>[2x]MNPAAEAEFNILLATDSYKVTHYKQYPPNTSKVYSYFECREKKTENSKLRKVKYEETVFY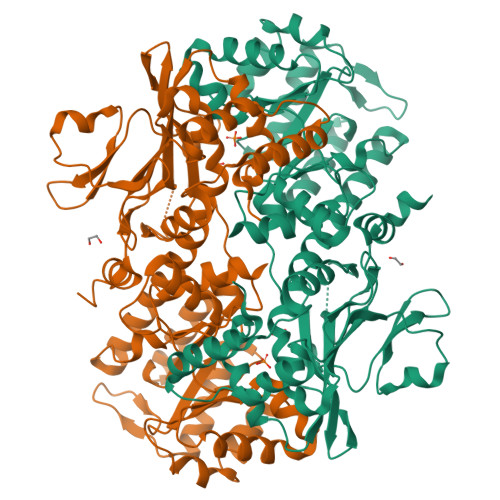GLQYILNKYLKGKVVTKEKIQEAKDVYKEHFQDDVFNEKGWNYILEKYDGHLPIEIKAVPEGFVIPRGNVLFTVENTDPECYWLTNWIETILVQSWYPITVATNSREQKKILAKYLLETSGNLDGLEYKLHDFGYRGVSSQETAGIGASAHLVNFKATDTVAGLALIKKYYGTKDPVPGYSVPAAEHSTITAWGKDHEKDAFEHIVTQFSSVPVSVVSDSYDIYNACEKIWGEDLRHLIVSRSTQAPLIIRPDSGNPLDTVLKVLEILGKKFPVTENSKGYKLLPPYLRVIQGDGVDINTLQEIVEGMKQKMWSIENIAFGSGGGLLQKLTRDLLNCSFKCSYVVTNGLGINVFKDPVADPNKRSKKGRLSLHRTPAGNFVTLEEGKGDLEEYGQDLLHTVFKNGKVTKSYSFDEIRKNAQLNIELEAAHHLEHHHHHHHH> MGSSHHHHHHAFHDVPSLGQKVGAGSQKDVFHSRQDPRQCICLFRPGTTGSIPAEQYAQKELETTKQLKNLGFPVVDAHALVKHQGSVGVAKD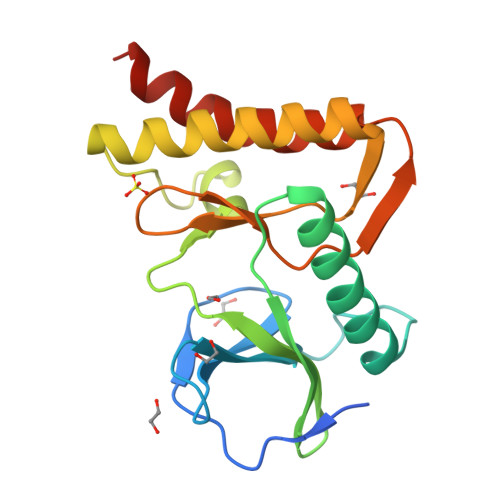FIHNALDSEDIVNNKKSLPDNLKFNKNVLEDCNAIIRRLKNLEVHIEDLQFLVDHNGHVLINDPRDVVRSSPDKSISKVNELRSHALNNLLDIDSD MLLs degrade N-acyl-L-homoserine lactones (AHLs), molecules that are used in a microbial communication system called quorum sensing (QS) to coordinate a variety of behaviors, including virulence and biofilm formation. We provide the structural and biochemical analysis of the lactonase GcL (WP_017434252.1), isolated from the thermophilic bacteria Parageobacillus caldoxylosilyticus. GcL is a thermostable, highly proficient lactonase with broad substrate specificity (kcat/KM values range between 104 to 106 M–1 s–1) for substrates such as N-butyryl (C4) L-homoserine lactone (HSL) and N-decanoyl (C10)-HSL. The binuclear center, common to all MLLs, is coordinated by five histidine residues and two aspartic acid residues.

We report here the kinetic characterization of several variants, including Ala157Gly, Ala157Ser, Gly156Pro and Ile237Met. While some of these variants show only modest changes in lactonase activity compared to the wild-type for several AHL substrates (e.g., Ile237Met), they show altered kinetics for specific substrates, resulting in changes in substrate preference. To gain some molecular insights into the effects of these substitutions on the active site configuration, structures were solved for both Gly156Pro and Ile237Met variants. On the other hand, the Ile237Met variant shows a slightly altered conformation of the Pro234-Asp240 loop, in the vicinity of the amide group of the AHL substrate. This conformational change is more distant from the atoms of a long acyl chain AHL substrate, and this is, therefore, consistent with the minimal changes in catalytic properties recorded for this variant. Following this, when considering the locations of the amino acid substitutions performed in the variants studied here, two of them (Tyr223Phe and Asp122Asn) are part of the first hydrophobic subsite where the lactone ring is accommodated, Ile237Met is located at the second hydrophobic subsite, and the rest (Gly156Pro, Ala157Gly and Ala157Ser) are located in the third hydrophilic subsite.

>[3x]WSHPQFEKENLYFQSMANVIKARPKLYVMDNGRMRMDKNWMIAMHNPATIHNPNAQTEFVEFPIYTVLIDHPEGKILFDTSCNPNSMGPQGRWAESTQQMFPWTATEECYLHNRLEQLKVRPEDIRYVVASHLHLDHAGCLEMFTNATIIVHEDEFNGALQCYARNQKEGAYIWADIDAWIKNNLQWRTVKRHEDNILLAEGVKVLNFGSGHAWGMLGLHVELPETGGIILASDAIYTAESYGPPIKPPGMIYDSLGYMNTVERIRRIAQETKSQVWFGHDAEQFKKFRKSTEGYYE> MSNSLEKKVSLLQNESVEKNKSIQSLHNQICSFEIEIERQKEMLRNNESKILHLQRVIDSQAEKLKELDKEIRPFRQNWEEADSMKSSVESLQNRVTELESVDKSAGQVARNTGLLESQLSRHDQMLSVHDIRLADMDLRFQVLETASYNGVLIWKIRDYKRRKQEAVMGKTLSLYSQPFYTGYFGYKMCARVYLNGDGMGKGTHLSLFFVIMRGEYDALLPWPFKQKVTLMLMDQGSSRRHLGDAFKPDPNSSSFKKPTGEMNIASGCPVFVAQTV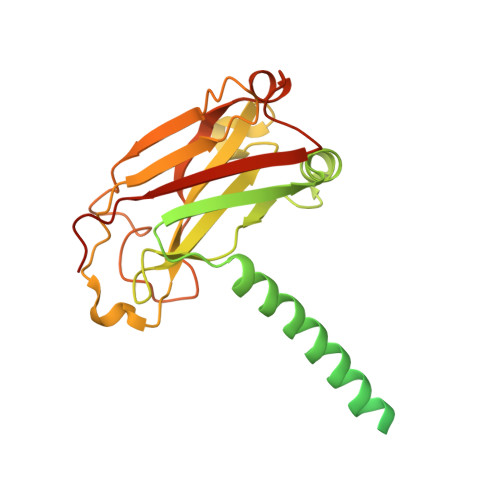LENGTYIKDDTIFIKVIVDTSDLPDPGGSLVPR>[2x]MTVTRPRAERGAFPPGTEHYGRSLLGAPLIWFPAPAASRESGLILAGTHGDENSSVVTLSCALRTLTPSLRRHHVVLCVNPDG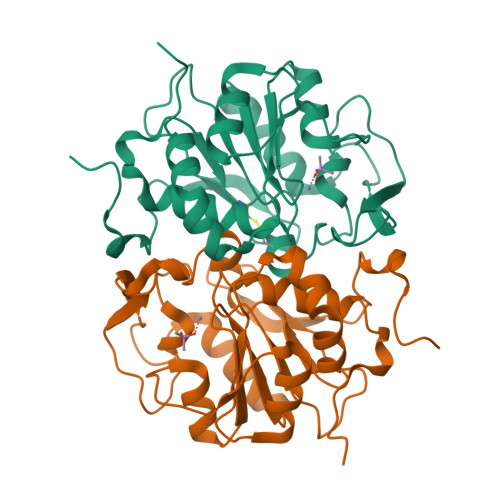CQLGLRANANGVDLNRNFPAANWKEGETVYRWNSAAEERDVVLLTGDKPGSEPETQALCQLIHRIQPAWVVSFHDPLACIEDPRHSELGEWLAQAFELPLVTSVGYETPGSFGSWCADLNLHCITAEFPPISSDEASEKYLFAMANLLRWHPKD>DADLATGAKVFSANCAACHAGGINLVNAEKTLKKEALEKFGMNSIVAITTQVTNGKAGMPAFKGRLTDDQIAAVAAYVLDQA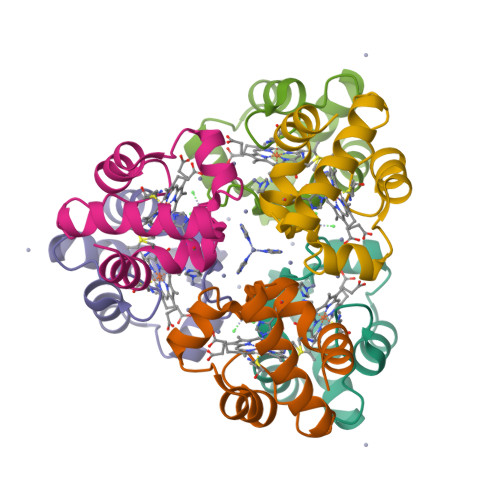EKGW[2x]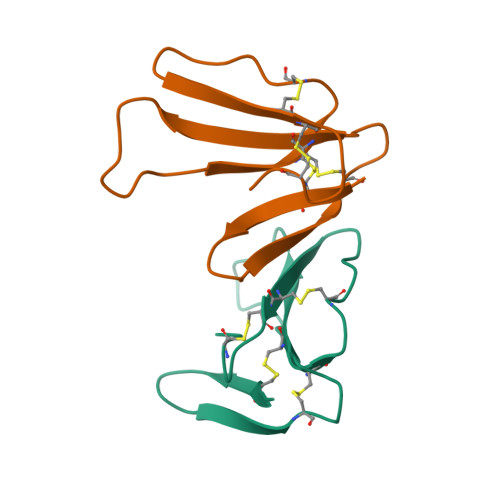>[3x]RLCLSDYSIFSETIEICPEGHNYCFKKFPKGITRLPWVIRGCAATCPKPEAQVYVDCCARDKCNR>MANLTEKFLRIFARRGKSIILAYDHGIEHGPADFMDNPDSADPEYILRLARDAGFDGVVFQRGIAEKYYDGSV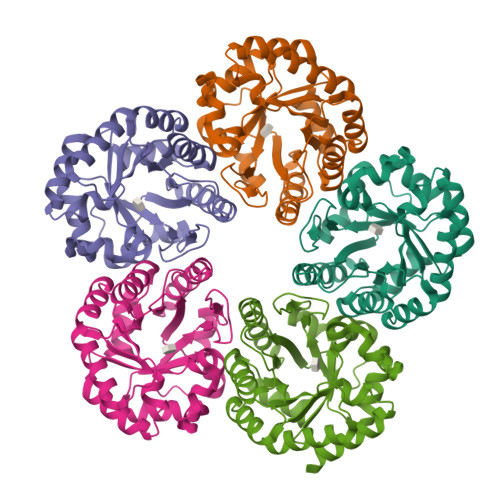PLILKLNGKTTLYNGEPVSVANCSVEEAVSLGASAVGYTIYPGSGFEWKMFEELARIKRDAVKFDLPLVVESFPRGGKVVNETAPEIVAYAARIALELGADAMKIKYTGDPKTFSWAVKVAGKVPVLMSGGPKTKTEEDFLKQVEGVLEAGALGIAVGRNVWQRRDALKFARALAELVYGGKKLAEPLNV[10x]> CFTPESTALLESGVRKPLGELSIGDRVLSMTANGQAVYSEV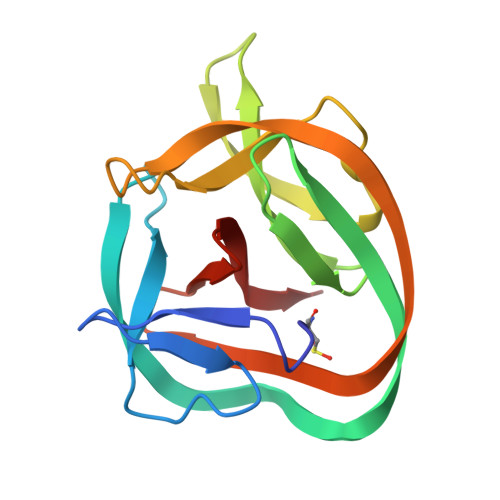ILFMHRNLEQMQNFVQLHTDGGAVLTVTPAHLVSVWQPESQKLTFVFADRIEEKNQVLVRDVETGELRPQRVVKVGSVRSKGVVAPLTREGTIVVNSVAASCYAV> LTCDQLPKAAINPIQEFIDSNPLEFEYVLTETFECTTRIYVQPARWSTTKAPTALDIKGTQ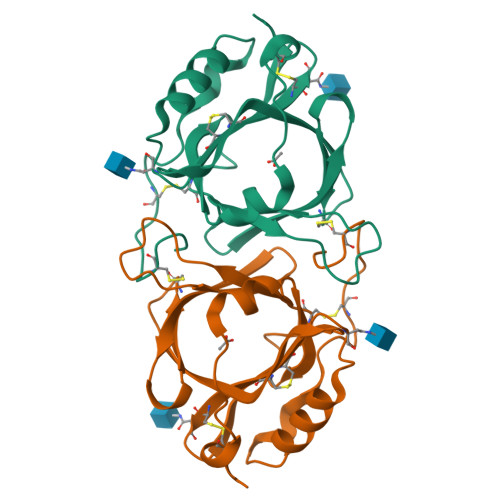IMAYDFVGGPENSAHLNECHTGDKQVWYFQYTNLLTDNGSSYCAYRCNGTEIIEYKCASNNNGTDPLQHQAMEVAKTVPNGDKIHYAKSNCPETHGCFAFY> MNNDDYPWFRKRGYLHFDEPVSLKKAVKYVSSPEKIIKHSFLPFLSFEVKSFKIKKDKSTKQLSKTEKLRPIAYSSHLDSHIYAFYAEYLTGHYELLIQENNLHENILAFRSLNKSNIEFAKRAFDTITEMGECSAVALDLSGFFDNLDHQILKHQWCKVIGTEALPQDHFAIYKSITRYSKVDKNRAYEILGISKNNPKYNRRKICTPVDFRNKIRKNGLIIVNNSQKGIPQGSPISALLSNIYMLDFDIEMRDYAQERGGHYYRYCDDMLFIVPTKYNKTLAGDVAQRIKHLKVELNTKKTEIRDFIYKDSTLVANMPLQYLGFIFDGSNILLRSSSLARYSERMKRGVRLAKATMDSKNRIRENKGEALKALFKKKLYARYSHIGRRNFLTYGYRAAKIMNSKAIKRQLKPLQKRLENEILK

Here, we show that in the DRT2 defense system the reverse transcriptase binds a neighboring pseudoknotted non-coding RNA. Upon bacteriophage infection, a template region of this RNA is reverse transcribed into an array of tandem repeats that reconstitute a promoter and open reading frame, allowing expression of a toxic repetitive protein and an abortive infection response. The system consists of a 280 nt ncRNA upstream of a gene for a 425 amino acid RT-domain protein with no additional domains. Our results demonstrate that upon phage infection, the DRT2 RT reverse transcribes the template region of the DRT2 ncRNA into a concatemeric repetitive ccDNA that then templates transcription (“forward transcription”) of the ccDNA into a repetitive neo mRNA that is then translated into a toxic Neo protein.

The region of the ncRNA 5′ to the template (“5′ handle”) forms a hairpin that docks into the finger-insertion domain. The 3′ region of the ncRNA downstream of the template is intricately folded and intimately associated with the elongated thumb domain of the RT. One long 34-nt hairpin (the “tower”) and a shorter 18-nt hairpin (the “buttress”) form A-minor motif interactions and rise against one side of the thumb, an interaction which is secured by a potassium ion-stabilized pseudoknot that wraps around the other side of the thumb. The rest of the template region is loosely bound to the RT, as evidenced by weaker cryo-EM density, but template bases 29–37 and 86–135 are visible as three helices forming a three-way junction. The final eight nucleotides of the template (bases 141–148) are visible within the RT active site. Strikingly, template bases 142–146 are already annealed to a 5-nt DNA primer “GATAT,” we therefore refer to these template bases as the primer-binding site (PBS). We conclude that the “GATAT” DNA primer is covalently linked to the 3′ end of the ncRNA and is synthesized by the DRT2 RT. The 5′ phosphate of the primer G and the 3′ oxygen of the ncRNA C278 (the last RNA base clearly resolved in the cryo-EM density) are separated by 11.7 Å, which would readily be bridged by two additional RNA bases. Instead, we saw that the incoming dNTP binding site is blocked by a guanosine nucleotide from the 3′ end of the ncRNA (G277) which forms a non-Watson-Crick pair with template base C141.>[2x]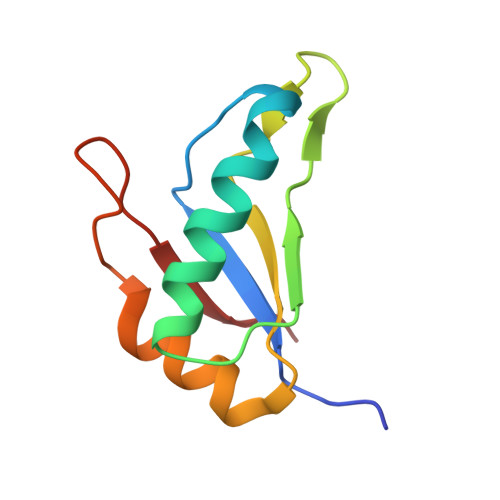GPLGSDQYIVVNGAPVIPSAKVPVLKKALTSLFSKAGKVVNMEFPIDEATGKTKGFLFVECGSMNDAKKIIKSFHGKRLDLKHRLFLYTMK>[8x]GSHMAKEEIIWESLSVDVGSQGNPGIVEYK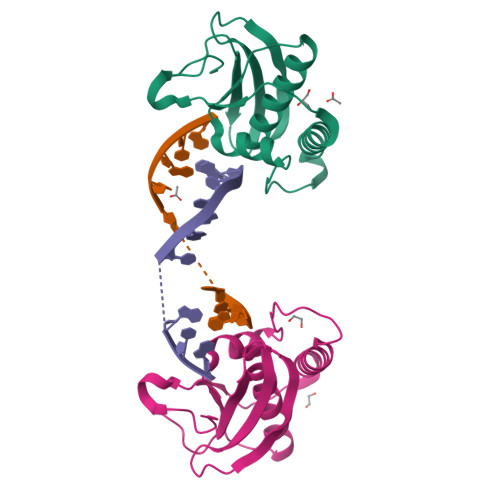GVDTKTGEVLFEREPIPIGTNNMGEFLAIVHGLRYLKERNSRKPIYSNSQTAIKWVKDKKAKSTLVRNEETALIWKLVDEAEEWLNTHTYETPILKWQTDKWGEIKADYGRK In this study, we report on the detailed structural and biochemical characteristics of an esterase (EaEST) from a psychrophilic bacterium Exiguobacterium antarcticum B7. The crystal structure of peracetate-bound EaEST was resolved at high resolution, revealing that EaEST retains the characteristic α/β-hydrolase fold with a cap domain and has a catalytic triad of Ser96, Asp220, and His248. Using an analytical ultracentrifugation (AUC) analysis, we also confirmed that the purified EaEST protein forms a stable trimer in solution. These studies provide insight into an unusual enzymatic feature, the dual catalytic role of EaEST as a typical esterase and perhydrolase. The results of analytical ultracentrifugation demonstrated that the purified EaEST protein is a stable trimer in solution.

The crystal structure of an esterase (EaEST) from Exiguobacterium antarcticum was determined in a P3 space group. The final model was refined up to 1.9 Å and produced Rwork and Rfree values of 0.185 and 0.235, respectively. The asymmetric unit of an EaEST crystal contains two protomers. During the process of structure determination, unknown electron-density maps were found near the active sites of both molecules in the asymmetric unit. Even if no specific ligands were added to EaEST at purification and crystallization, the unknown electron density was initially interpreted as an acetate because of crystallization conditions containing 0.2 M ammonium acetate. After building and refining the model, additional electron density was clearly observed in the hydroxyl group of acetic acid, indicating that EaEST has perhydrolysis activity via acetic acid. Using repetitive refinement, the peracetate molecule was perfectly fitted into the electron-density map. The hydroxyl group of peracetic acid forms hydrogen bonds with the O atom of Ser96, the NE2 atom of His248, and main-chain oxygen atom of Trp30. The active site of EaEST is comprised of a conserved catalytic triad (Ser96, Asp220, and His248) and the neighboring hydrophobic pocket, which is composed of the hydrophobic residues Trp30, Phe127, Met137, Leu145, Met156, Phe160, Ile163, Leu199, Phe164, and Val 222. The crystal structure of EaEST in peracetate-bound form provides the first structural insights into the final product-bound state during perhydrolysis.

>[2x]MGTFIQAVDGTKIYVEDIGSGQPVVMLHGWPANNNMFEYQKNRLLEEGYRYIGVDYRGYGKSDAPATGYDYTTMASDINEVIQQLKLTNVTLLGFSMGGGIALKYLLNHGESNVSKLILAGAAAPVFTQRDGYPYGMTKDEVDALIEDTKQDRPSMLKGFGEIFFAKEHPEPLQQWFHNLSVDASSHGTIQSAIALRDEDLRDGLPKITVDTLIMHGKKDQVCPFEFAEVMHENIAGSRLEVFEESGHGMFLDEREKFTETLVSYVKSSQTV>MVKLAEFSRTATFAWSHDKIPLLVSGTVSGTVDANFSTDSSLELWSLLAADSEKPIASLQVDSKFNDLDWSHNNKIIAGALDNGSLELYSTNEANNAINSMARFSNHSSSVKTVKFNAKQDNVLASGGNNGEIFIWDMNKCTESPSNYTPLTPGQSMSSVDEVISLAWNQSLAHVFASAGSSNFASIWDLKAKKEVIHLSYTSPNSGIKQQLSVVEWHPKNSTRVATATGSDNDPSILIWDLRNANTPLQTLNQGHQKGILSLDWCHQDEHLLLSSGRDNTVLLWNPESAEQLSQFPARGNWCFKTKFAPEAPDLFACASFDNKIEVQTLQNLTNTLDEQETETKQQESETDFWNNVSREESKEKPTVFHLQAPTWYGEPSPAAHWAFGGKLVQITPDGKGVSITNPKISGLESNTTLSEALKTKDFKPLINQRLVKVIDDVNEEDWNLLEKLSMDGTEEFLKEALAFDNDESDAQDDANNEKEDDGEEFFQQIETNFQPEGDFSLSGNIEQTISKNLVSGNIKSAVKNSLENDLLMEAMVIALDSNNERLKESVKNAYFAKYGSKSSLSRILYSISKREVDDLVENLDVSQWKFISKAIQNLYPNDIAQRNEMLIKLGDRLKENGHRQDSLTLYLAAGSLDKVASIWLSEFPDLEDKLKKDNKTIYEAHSECLTEFIERFTVFSNFINGSSTINNEQLIAKFLEFINLTTSTGNFELATEFLNSLPSDNEEVKTEKARVLIASGKSLPAQNPATATTSKAKYTNAKTNKNVPVLPTPGMPSTTSIPSMQAPFYGMTPGASANALPPKPYVPATTTSAPVHTEGKYAPPSQPSMASPFVNKTNSSTRLNSFAPPPNPYATATVPATNVSTTSIPQNTFAPIQPGMPIMGDYNAQSSSIPSQPPINAVSGQTPHLNRKANDGWNDLPLKVKEKPSRAKAVSVAPPNILSTPTPLNGIPANAASTMPPPPLSRAPSSVSMVSPPPLHKNSRVPSLVATSESPRASISNPYAPPQSSQQFPIGTISTANQTSNTAQVASSNPYAPPPQQRVATPLSGGVPPAPLPKASNPYAPTATTQPNGSSYPPTGPYTNNHTMTSPPPVFNKPPTGPPPISMKKRSNKLASIEQNPSQGATYPPTLSSSASPLQPSQPPTLASQVNTSAENVSHEIPADQQPIVDFL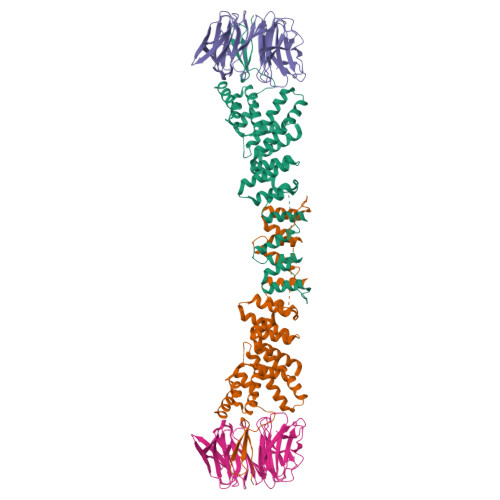KEELARVTPLTPKEYSKQLKDCDKRLKILFYHLEKQDLLTQPTIDCLHDLVALMKEKKYKEAMVIHANIATNHAQEGGNWLTGVKRLIGIAEATLN[2x];>[2x]MVVIANAHNELIHDAVLDYYGKRLATCSSDKTIKIFEVEGETHKLIDTLTGHEGPVWRVDWAHPKFGTILASCSYDGKVLIWKEENGRWSQIAVHAVHSASVNSVQWAPHEYGPLLLVASSDGKVSVVEFKENGTTSPIIIDAHAIGVNSASWAPATIEEDGEHNGTKESRKFVTGGADNLVKIWKYNSDAQTYVLESTLEGHSDWVRDVAWSPTVLLRSYLASVSQDRTCIIWTQDNEQGPWKKTLLKEEKFPDVLWRASWSLSGNVLALSGGDNKVTLWKENLEGKWEPAGEVHQ>[2x]GSARLKGITLRIGVIESVPFTIVANVIDTSGRNT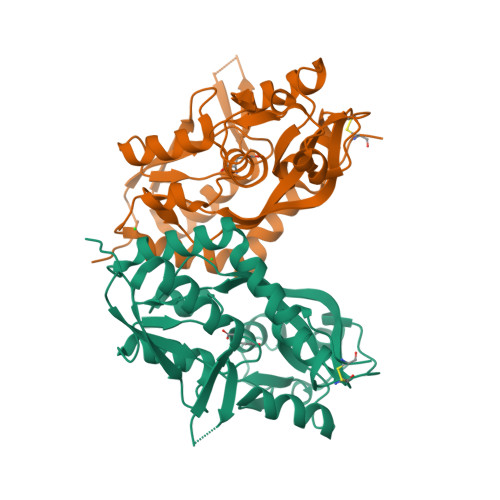TKLTGYVLDLIEYLRDKMGFVADVQLAPPNTSYTGLVLALANGDYDIAIGDITVTSARREIVAFSNSISDNSMRILMRKGTLIDGMDDLKNGKIPYNRIGIRIGTAGEDYYLREISGGSRNFYPLKSRQEMYDSLLAGIIDVSFMDIGTAEYVTNNIYCNLTLVGEDFDKSTFGIVTPKEWLYAKDLDVNILSLRETGILDNLKKKWFQTKACP> TSSINFLTSDDDASAAAMEAFIGTNHHSSLFPPPPQQPPQPQFNEDTLQQRLQALIESAGENWTYAIFWQISHDFDSSTGDNTVILGWGDGYYKGEEDKEKK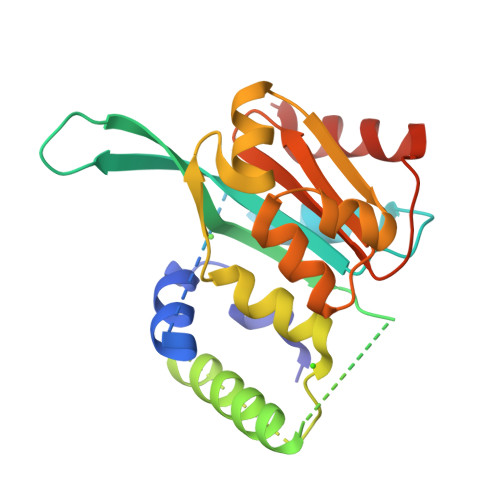KNNTNTAEQEHRKRVIRELNSLISGGIGVSDESNDEEVTDTEWFFLVSMTQSFVNGVGLPGESFLNSRVIWLSGSGALTGSGCERAGQGQIYGLKTMVCIATQNGVVELGSSEVISQSSDLMHKVNNLFNFNNGGG4-(4-{[(5R)-2,4-dioxo-1,3-thiazolidin-5-yl]methyl}-2-methoxyphenoxy)-3-(trifluoromethyl)benzonitrile | C19 H13 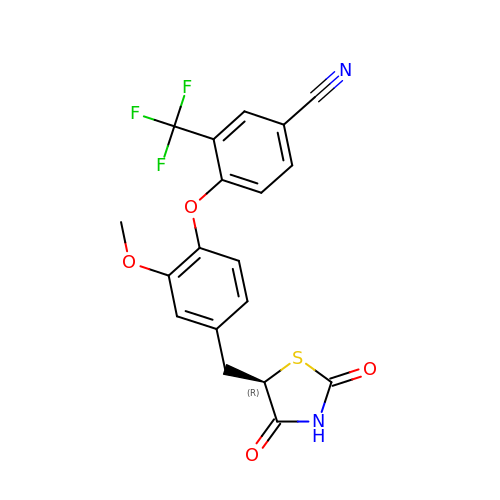F3 N2 O4 S | IOTPZQVXYNGZSS-MRXNPFEDSA-N>MSQRITIDPVTRIEGHLRIDCEIENGVVSKAWASGTMWRGMEEIVKNRDPRDAWMIVQRICGVCTTTHAISSVRAAESALNIDVPVNAQYIRNIILAAHTTHDHIVHFYQLSALDWVDITSALKADPAKASAMLNGVSTWHLNSAEEFTKVQNKIKDLVASGQLGIFANGCWGHPAMQLPPEVNLIAVAHYLQALECQRDANRVVALLGGKTPHIQNLAVGGVANPINLDGLGVLNLERLMYIKSFIDKLSDFVEQVYKVDTAVIAAFYPEWLERGQGAVNYLSAPEFPTDGKNGSFLFPGGYITDADLSTYRPITSHSDEYLIKGIQESAKHAWYKDEAPQAPWEGTTVPDYTGWSDDGKYSWVKAPTFYGKTVEVGPLANMLCKLAAKRESTHAKLNEIVAIYTKLTGKTIEVAQLHSTLGRIIGRTVHCCELQNVLQDQYNALIVNIGKGDHTTFVKPDIPATGEFKGVGFLEAPRGMLSHWMVIKDGIISNYQAVVPSTWNSGPRNFNDEVGPYERSLVGTPIADPNKPLEVVRTIHSFDPCMSCAVHVVDVDGNEVVSVKVL[2x];>[2x]EMAESVSRPQRPPVIWIGAQECTGCTESLLRATHPTVENLVLETISLEYHEVLSAAFGHQVEENKHNALEKYKG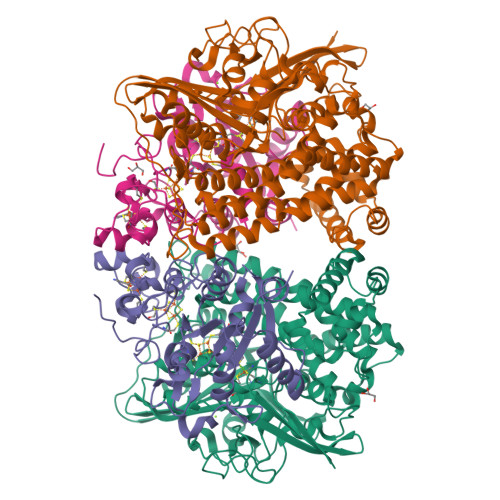QYVLVVDGSIPLKDNGIYCMVAGEPIVDHIRRAAEGAAAIIAIGSCAAWGGVAAAGVNPTGAVGLQEVLPGKTIINIPGCPPNPHNFLATVAHIITYGKPPKLDAKNRPTFAYGRLIHEHCERRPHFDAGRFAKEFGDEGHREGWCLYHLGCKGPETYGNCSTLQFCDVGGVWPVAIGHPCYGCNEEGIGFHKGIHQLAHVENQTPRSEKPDVNIKEGGNISAGAVGLLGGVVGLVAGVSVMAVRELGRQQKKDNADSRGE> GLAEKLVPAKKVKNGVLYKSGHIKVSNVRCSYPHLDKPYGGEDGGEPKYSITLLMPKDTHGAIKKIIDEQIEL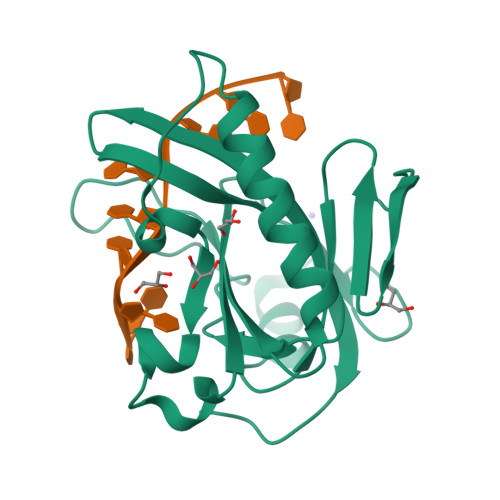TKKNHKTGALKVAPSMLFIKDGDVDFPDKPECEGMWVISARESTRPDVLNMEREELESPNEIAEEIYGGCWVSSVIRPWSQENKYGKRINANLLSVLKRKDDEPFGE N-(tert-butoxycarbonyl)-L-alanyl-N-[(1R)-1-(carboxyamino)-2-phenylethyl]-L-prolinamide 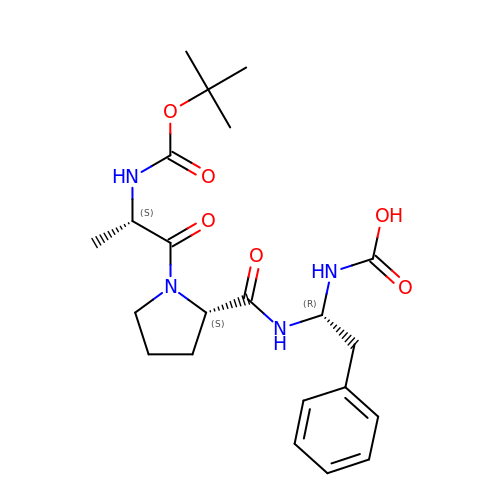| C22 H32 N4 O6 | YLCJIHHAPKJGHH-BHYGNILZSA-N>MSSCKDSLSLMAMWGSIARFDPKHERSFEGPEKRLEVIMRVVDGTHVSGLLAHDDDVWQKVIDAICAHIVSREFNEYIRSYVLSE[2x];>[2x]XSLFVMKDRVILITCGTITLLNCVPLICEAVSTVCGEVEWVSFMHKNYSFPWEQKGPHLSMAEEFKTLRSHFPSGQPFIFGPIDSDHYFLYFHSDVVQPSCSDDAQLSMTMYGLDRNQTKHWYSDKMLPTGPETAVIREATGLSEVVDDSWILHDLQYEPCGYSINAIRGSEYQTIHITPEEHCSFASYETNTCALNYSKCICGVLRVFDPERFSVIVFIDPDSAVGKSYHSGGTIGVEPEYYPNYEAHHRTVNEYTPGHWVLKVNYVKRAVGTVGTSAASGAKE;>[2x]MSVTRINQQTECPSSVHDLVSCWGGCTQSKTSTDSGLEKRFELNFAQPVDIGTVTVKQLASVMERAGESLRQNSAELGIHTLKFDRSLLVFTAKQIVVRSSVSVMLHEAVHPMLELMRSHNIIVDWASFMRVNYGSPWDMTSETSDIMAHEYAELKSAFPTGHPYLAGPVDRDHCFYFVYDGIDRDPSSCRRENDVQINVYMYNVQADDEYDLDGNTKEQQLLVSHCAGEYETLRVSTYGSTHPFASFETNA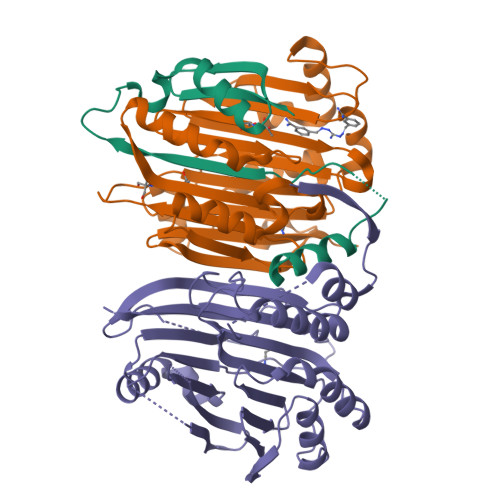VSAASDITKIVNGLLKKFYPERVLLVLLQDRDAQGTTACGVMDRLEGFTVVHRGANHFGGGYVFHQATYARSA>GSHMSAPLPLDELRTFAEVLDRVKAAYVEPVDDKTLLENAIKGMLSNLDPHSAYLGPEDFAELQESTSGEFGGLGIEVGSEDGFIKVVSPIDDTPAARAGIQPGDLIVQIDGKPTKGQSMTEAVDSMRGKAGSPITLTIVRDGGRPFDVELKRAIIKVKSVKSQVLEPGYAYLRITQFQVNTGEEVVKALNQLRKDNKGRLKGLVLDLRNNPGGVLQSAVEVADAFLTKGLIVYTKGRIANSELRFSADPADPSDKVPLVVLINGGSAAAAEIVAGALQDQKRAILMGTDSFGKGSVQTVLPLNNDRALKLTTALYYTPNGRSIQAQGIVPDIEVGRAKVTQERSSFEGFKEADLQGHLANGNGGADRPTGKRAAPSERPQDSDYQLSQALSLLKGLSVTRGN[3x];> MEDTAVETKAKPEKYGSFSEDSLYSLLVAELAGQRNRFDIALSNYVVQAQKTRDPGVSERAFRIAEYLGADQEALDTSLLWARSAPDNLDAQRAAAIQLARAGRYEESMVYMEKVLNGQGDTHFDFLALSAAETDPDTRAGLLQSFDHLLKKYPNNGQLLFGKALLLQQDGRPDEALTLLEDNSASRHEVAPLLLRSRLLQSMKRSDEALPLLKAGIKEHPDDKRVRLAYARLLVEQNRLDDAKAEFAGLVQQFPDDDDLRFSLALVCLEAQAWDEARIYLEELVERDSHVDAAHFNLGRLAEEQKDTARALDEYAQVGPGNDFLPAQLRQTDVLLKAGRVDEAAQRLDKARSEQPDYAIQLYLIEAEALSNNDQQEKAWQAIQEGLKQYPEDLNLLYTRSMLAEKRNDLAQMEKDLRFVIAREPDNAMALNALGYTLADRTTRYGEARELILKAHKLNPDDPAILDSMGWINYRQGKLADAERYLRQALQRYPDHEVAAHLGEVLWAQGRQGDARAIWREYLDKQPDSDVLRRTIKRLTGAETP

During bacterial cell growth, hydrolases cleave peptide cross-links between strands of the peptidoglycan sacculus to allow new strand insertion. The Pseudomonas aeruginosa carboxyl-terminal processing protease (CTP) CtpA regulates some of these hydrolases by degrading them. CtpA assembles as an inactive hexamer composed of a trimer-of-dimers, but its lipoprotein binding partner LbcA activates CtpA by an unknown mechanism. LbcA has an N-terminal adaptor domain that binds to CtpA, and a C-terminal superhelical tetratricopeptide repeat domain.

The LbcA density in the CtpA–LbcA EM map thickens in the middle of the TPR region, suggesting that the TPR domain may fluctuate in multiple conformations. Therefore, we performed a heterogeneous refinement leading to two CtpA–LbcA EM maps. As expected, the two CtpA hexamers in the two 3D maps are superimposable but the two LbcA supercoils are wide apart, with one supercoil in a higher position remote to the front CtpA and the other in a lower position proximal to the front CtpA. We next performed focused refinement in the top one-third region of the two maps and derived two local EM maps at around 4 Å resolution. We found that in these two local structures, the LbcA adaptor domain (H1–H6) binds to CtpA in essentially the same binding mode, and the difference between the two structures is limited to the LbcA TPR domain, which is 44 Å and 18 Å, respectively, above the front CtpA. However, both conformations were in complex with active CtpA, implying that the two positions of the superhelical TPR domain have no effect on the allosteric activation mechanism. To bring the C-termini of these substrates to the CtpA substrate binding tunnel, the TPR domain of LbcA needs to be configured flexibly to accommodate the substrates with different sizes.>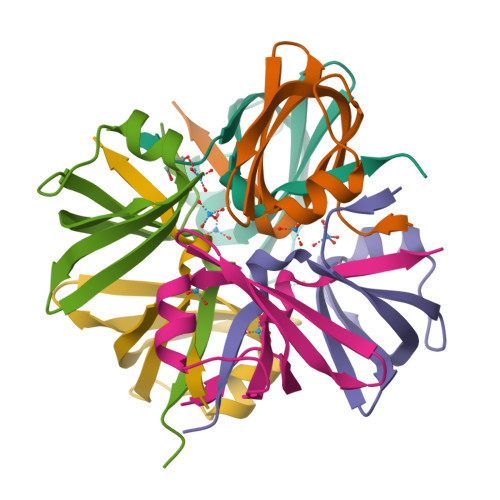MKLSARNQLAGKVVSIKEGAVNGIVVLDIGGGNQISSTISMDSIRELGLQVGSDAYAVIKATSVMIGIDDWSHPQFEK[6x]>HMVYPTTLHIIGGQGGNAFSFNGQENAATLQKLSVSVGGWQVRGVQVWLTDGRRETFGAMDSSAKEFEFESGEFIKSLSLWGNGAGTRLGAIKFITSRSREFFAKMTDWGLKTEYKIDVGSGICLGVQGRGGSDIDSMGFIFINAIKSSVIQDMKYPTMHQILPNVQMEEIKEMEYKNDTSIVQSYT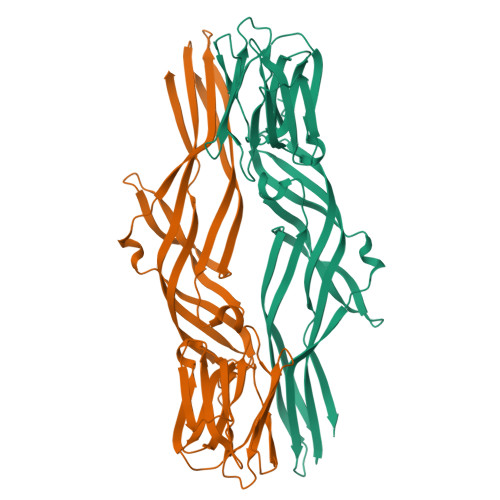FESSKKIIKKSSWSTTNKIESTFSLSVKAGIPEVMEVETGFSFTVGSESTHAVEESEEKTETLTFPVTVPTHKTVTVVANIGRADIDLPYTALLRITCVNGASLDAPLSGIYKGLTYTKMTAVATES[2x]>MYKPEQLLIFTTCPDADIACRIATALVEAKLAACVQIGQAVESIYQWDNNICQSHEVPMQIKCMTTDYP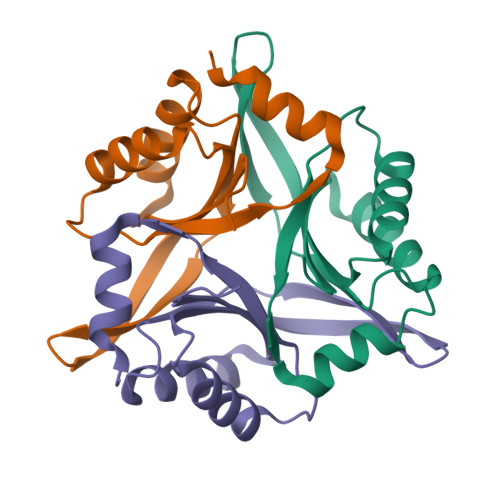AIEQLVITMHPYEVPEFIATPIIGGFGPYLQWIKDNSPS[6x]> MISSYYFGAISLILIGLYAVLVKKNLLKILIGLSIMETGVNLLLISIGYVSGKSAPILSEGVTASNAVDPIPQAL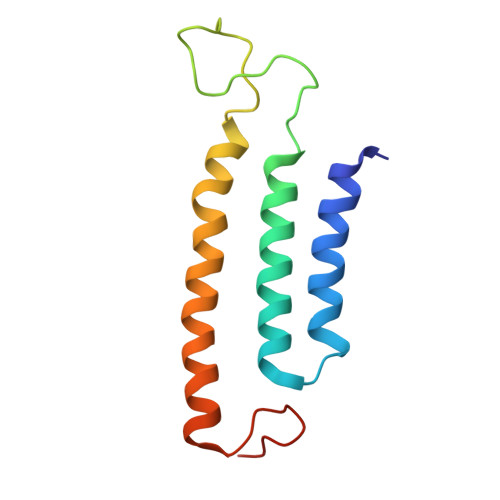VLTAIVIGVATTAMALSVAILLYEKYGTLNIEEIRRLRG>MYRYEKKGPKRGVALYSYSAEFGLTKTLEDCFEDLHDMGAHGIEILANTHIENYPYPTDEWVEKWWRLCDKYEIVPVEYGNWIDSHVLGDRDLTTEESVEMLKRDIRLAHRLGFTVMRTKMPVINDLLEPVENWKEIIKGALPLAEELGIKMCPEIHTPSNLKGKLVNDFVEFIKETGTKNFGLNIDFSVFRTSFAEGEWVDPNYTPNKPEDIIPLLPYVYCCHAKFIHMSDDFKETTIPYEEVVKTMEDNGYEGYLLSEYEGADKYDEGYEVGQTLRKHHILLKNLLGD[4x];>MEKQVIQSVGFRNIKNGNGEITG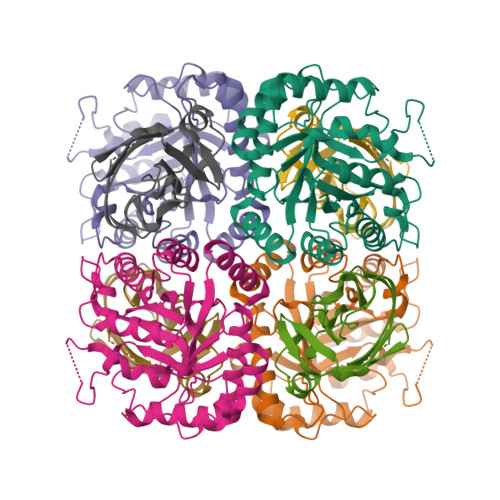FQFKVKLPYYRGVFLSQIRPGTLFVDGQKIEKDQITWTINGEEYTNQEMRGDFKTHWATTKPAVLKVKMPGGLAQGYHDLKYGFCFTSSYMPPIIQDGLDPDKESMVYMPEFGHHVNERRLLIVKLAAALEHHHHHH[4x]>MRCIGISNRDFVEGVSGGSWVDIVLEHGSCVTTMAKNKPT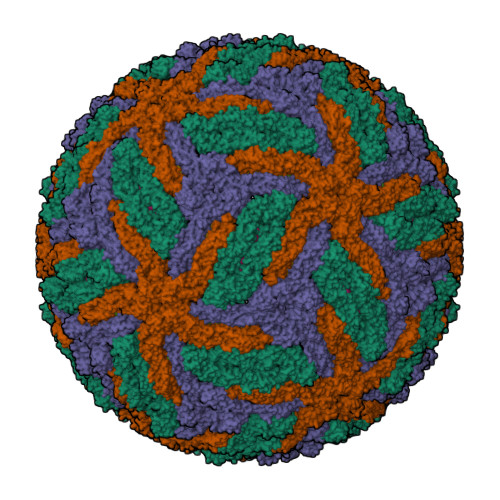LDFELIETEAKQPATLRKYCIEAKLTNTTTDSRCPTQGEPSLNEEQDKRFVCKHSMVDRGWGNGCGLFGKGGIVTCAMFTCKKNMKGKVVQPENLEYTIVITPHSGEEHAVGNDTGKHGKEIKITPQSSITEAELTGYGTVTMECSPRTGLDFNEMVLLQMENKAWLVHRQWFLDLPLPWLPGADTQGSNWIQKETLVTFKNPHAKKQDVVVLGSQEGAMHTALTGATEIQMSSGNLLFTGHLKCRLRMDKLQLKGMSYSMCTGKFKVVKEIAETQHGTIVIRVQYEGDGSPCKIPFEIMDLEKRHVLGRLITVNPIVTEKDSPVNIEAEPPFGDSYIIIGVEPGQLKLNWFKKGSSIGQMIETTMRGAKRMAILGDTAWDFGSLGGVFTSIGKALHQVFGAIYGAAFSGVSWIMKILIGVIITWIGMNSRSTSLSVSLVLVGVVTLYLGVMVQA[3x];>SVALVPHVGMGLETATETWMSSEGAWKHAQRIETWILRHPGFTIMAAILAYTIGTTHFQRALIFILLTAVAPSMT[3x]>GGAHKVRAGGPGLERAEAGVPAEFSIWTREAGAGGLAIAVEGPSKAEISFEDRKDGSCGVAYVVQEPGDYEVSVKF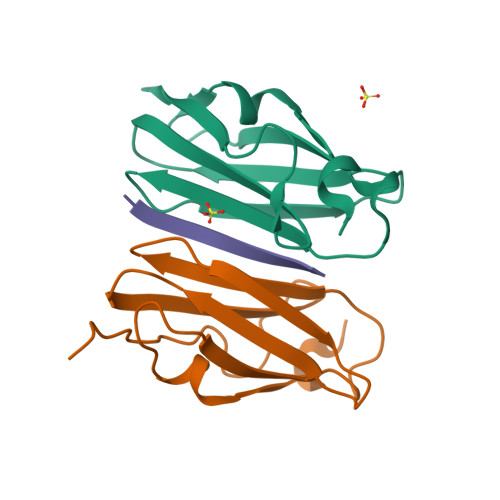NEEHIPDSPFVVPVASPS[2x];> PEKRVASSVFITLAP> GHMDVGERSSDQGTTVLTEAQ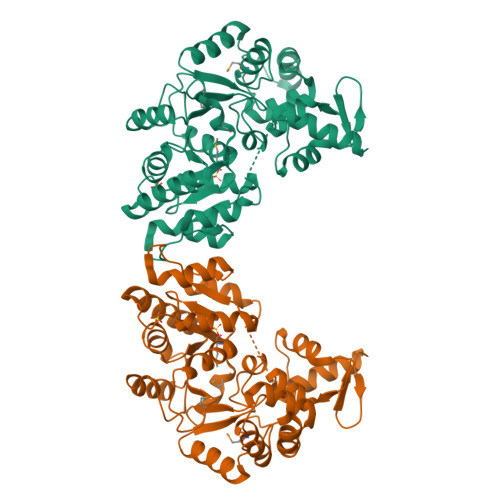RIDWMRLIRAENVGPRTFRSLINHFGSARAALERLPELARRGGAARAGRIPSEDEARREIEAGRRIGVELVAPGETGYPTRLATIDDAPPLLGVHALPEALAVMARPMIAIVGSRNASGAGLKFAGQLAADLGAAGFVVISGLARGIDQAAHRASLSSGTVAVLAGGHDKIYPAEHEDLLLDIIQTRGAAISEMPLGHVPRGKDFPRRNRLISGASVGVAVIEAAYRSGSLITARRAADQGREVFAVPGSPLDPRAAGTNDLIKQGATLITSASDIVEAVASILERPIELPGREPEHAPPEGEPDTGDRTRILALLGPSPVGIDDLIRLSGISPAVVRTILLELELAGRLERHGGSLVSLS> GGACAUAUAUACGCGU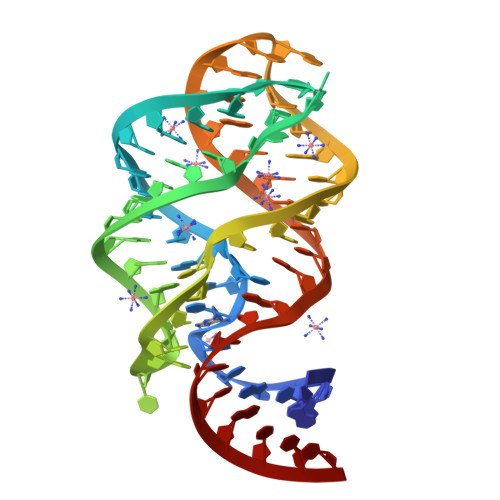GGAUAUGGCACGCGAGUUUCUACCGGGCACCGUAAAUGUCCGAUUAUGUCC>VPAFLGNLWALVGDPGTDHLIRWSPSGTSFLVSDQSRFAKEVLPQYFKHSNMASFVRQLNMYGFRKVVSIEQGGLLRPERDHVEFQHPSFVRGREQL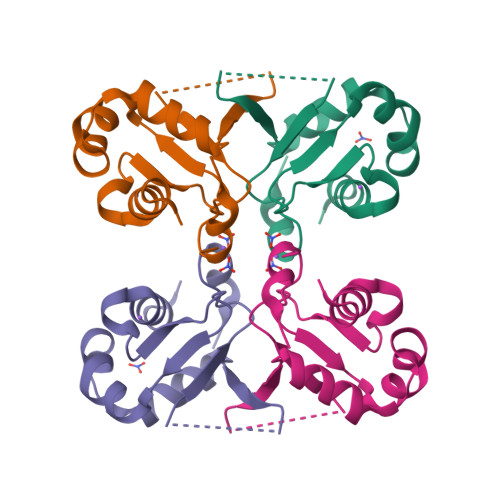LERVRRKV[2x]>[4x]KALDLKDITSGRFRPENIQGVIPMPDGEHYTQMSADGTQIIKYSFRTGEKVEVIFDVNQARECDFKNFDSYQFSPDGD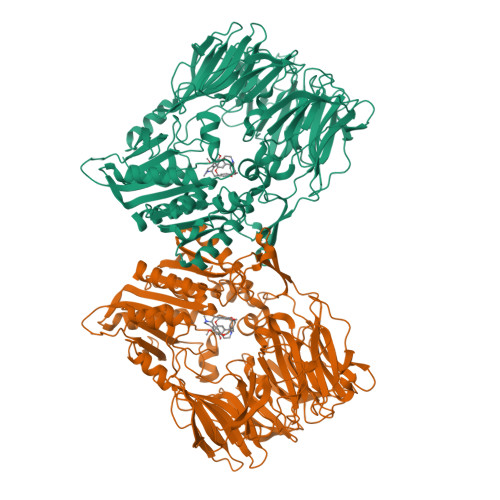KLLIATRTTPIYRHSYTAVHYIYPLKRNDKGVTTNNIIERLSDGGPQQVPVFSPDGTMIAFVRDNNIFLVKLLYGNSESQVTEDGKQNSVLNGIPDWVYEEEFGFNRALEFSADNTMIAFIRFDESEVPSYSFPMFAGEAPQITPLKDYPGEYTYKYPKAGYPNSKVEVRTYDIKSHVTRTMKLPIDADGYIPRIRFTKDASKLAVMTLNRHQDRFDLYFADPRSTLCKLVLRDESPYYIKENVFDNIKFYPETFSLLSERDGFSHLYWYSMGGNLIKKVTNGKYEVKDFLGYDEADGSFYYTSNEESPLRKAVYKIDKKGKKLKLSQREGTNTPLFSQSMKYYMNKFSNLDTPMLVTLNDNTGKTLKTLINNDQLKQTLSGYAIPQKEFFTFQTTDGVTLNGWMMKPANFSTSKKYPVLMYQYSGPGSQQVLDTWGISWETYMASLGYIVVCVDGRGTGGRGEAFEKCTYLKIGVKEAKDQVETALYLGKQPYVDKDRIGIWGWSYGGYMTLMSMSEGTPVFKAGVAVAAPTDWRFYDTIYTERFMRTPKENAEGYKESSAFTRADKLHGNLLLVHGMADDNVHFQNCAEYAEHLVQLGKQFDMQVYTNRNHGIYGGNTRQHLYTRLTNFFLNNL> GMRVLIVEDEPYLAEAIRDGLRLEAIAADIAGDGDTALELLSVNAYDIAVLDRDIPGPSGDEIAERIVASGSGMPILMLTAADRLDDKASGFGLGADDYLTKPFELQELALRLRALDRRRAHSRPPVREIAGLRLDPFRREVYRGGRYVALTRK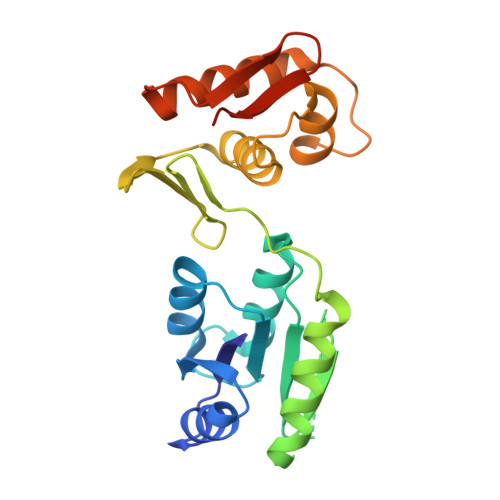QFAVLEVLVAAEGGVVSAEELLERAWDENADPFTNAVRITVSALRKRLGEPGIIATVPGVGYRIDTAPVSEQAGGDGG>GAMGSMKPYLFDLKLKDTEKLDWKKGLSSYLKKSYGSSQWRTFYDEKATSELDHLRNNANGELAPSSLSEQNLKYYSFLEHLYFRLGSKGSRLKMDFTWYDAEYSSAQKGLKYTQHTLAFEKSCTLFNIAVIFTQIARENINEDYKNSIANLTKAFSCFEYLSENFLNSPSVDLQSENTRFLANICHAEAQELFVLKLLNDQISSKQYTLISKLSRATCNLFQKCHDFMKEIDDDVAIYGEPKWKTTVTCKLHFYKSLSAYYHGLHLEEENRVGEAIAFLDFSMQQLISSLPFKTWLVE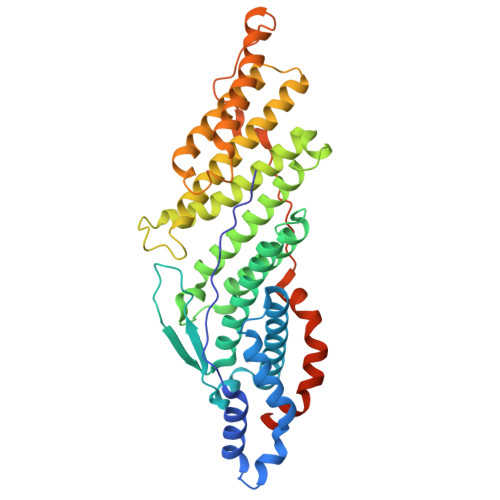FIDFDGFKETLEKKQKELIKDNDFIYHESVPAVVQVDSIKALDAIKSPTWEKILEPYMQDVANKYDSLYRGIIPLDVYEKESIYSEEKATLLR[2x]Here, we conduct a comprehensive functional analysis of the Antibiotic_NAT family of aminoglycoside acetyltransferases. AG resistance is primarily conferred by three classes of aminoglycoside-modifying enzymes (AMEs): phosphotransferases (APHs), nucleotidylyltransferases (ANTs), and acetyltransferases (AACs). AMEs permanently alter the AG substrate, preventing them from binding to their target, the A-site of the 16S rRNA in the bacterial ribosome. The fold typical of the Antibiotic_NAT family is evident in all structures, composed of 13 α-helices and 8 β-strands, and determined structures superpose with pairwise RMSD’s 0.8–1.0 Å between 197 to 266 matching Cα atoms.

To understand the structural basis of the highly promiscuous nature of group 1 Antibiotic_NAT enzymes, we pursued structural characterization of the AAC(3)-IVa representative of this clade in complex with AG substrates. To increase the chances of capturing substrate-bound enzyme complex we used the catalytically impaired His154Ala mutant of AAC(3)-IVa. Using this strategy, we were able to determine the crystal structures of AAC(3)-IVa enzyme in complex with gentamicin or apramycin to 2.6 and 2.8 Å, respectively. In both complex structures, the electron density corresponding to the AG molecule localized to the cleft between the major and minor subdomains of the enzyme. In the complex structures, the gentamicin molecule spans across the enzyme’s minor subdomain while the apramycin molecule is twisted nearly 90° relative to gentamicin. Additionally, Glu185 appears to be a critical residue for interactions with gentamicin and apramycin as it positions the 2-deoxystreptamine ring for modification through interactions with the 1-N of gentamicin or the 5-hydroxyl of apramycin. Interestingly, Cys190, which is just N-terminal to the Zn2+ binding site, interacts with the 3-N of gentamicin. The analysis of the AAC(3)-IVa•gentamicin complex allowed us to propose a mechanism for this enzyme’s ability to recognize 4,5-disubstituted AGs. In the complex structure, gentamicin’s 5-OH pointed out of the enzyme’s active site. If similarly oriented, 4,5-disubstituted AGs would not cause a steric clash with this enzyme’s active site.

>[6x]GQQMMQYEWRKAELIGQLLNLGVTPGGVLLVHSSFRSVRPLEDGPLGLIEALRAALGPGGTLVMPSWSGLDDEPFDPATSPVTPDLGVVSDTFWRLPNVKRSAHPFAFAAAGPQAEQIISDPLPLPPHSPASPVARVHELDGQVLLLGVGHDANTTLALAELMAKVPYGVPRHCTILQDGKLVRVDYLENDHCCERFALADRWLKEKSLQKEGPVGHAFARLIRSRDIVATALGQLGRDPLIFLHPPEAGCEECDAARQSIG>[2x]AR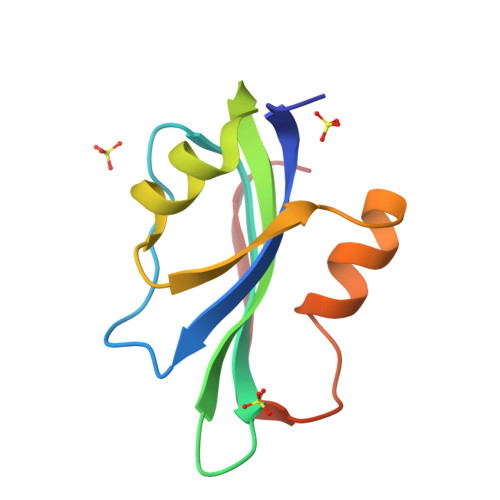QVICWCFTLNNPLSPLSLHDSMKYLVYQTEQGEAGNIHFQGYIEMKKRTSLAGMKKLIPGAHFEKRRGTQGEARAYSMKEDTRLEGPWEYGEL> LPQRWVSAGGSLSEWVVALGGESKLVGVDTTSQHPQALKQLPSVGYQRQLAAEGVLALRPDILIGTEEMGPPPVLKQLEGAGVRVETLSAKPDLEALESNLKKLGDWLGVPQRAEAAELDYRQRLRRQADWIAAAQKSQPAPGVLLVIGNAGGQLLVAGRNTGGDWVLNRAGARNLATHEGYKPISVEALAALDPVAVVIADRSLEGDAARAALL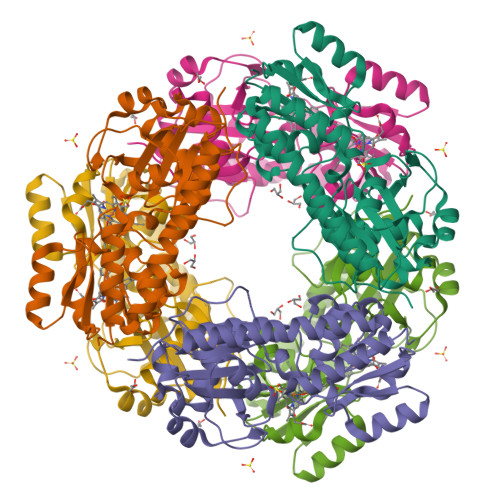KQNPGLAPTRAARDGRLLVLDPTLLVGGLGPRLPDGLAALSAAFYPSAKPLSTEAAHPLLGDDSTRTG Aminoacyl-tRNA synthetases catalyze aminoacylation of tRNAs with their cognate amino acids in two stages. First, the amino acid is activated by ATP to yield the AMP-activated amino acid, with loss of pyrophosphate, followed by transfer of the amino acid onto the tRNA. Malaria parasite genomes encode two different lysyl-tRNA synthetases (KRSs) that play a role in translation in either the cytoplasm (PfKRS1) or in the apicoplast (PfKRS2), while Cryptosporidium parasites and humans encode one copy. We present a selective inhibitor of both Plasmodium and Cryptosporidium lysyl-tRNA synthetase capable of clearing parasites from mouse models of malaria and cryptosporidiosis infection.

By using the luciferase ATP consumption (Kinase-Glo) assay platform with sub-Km substrate concentrations (thus biasing the assay toward identifying ATP-competitive inhibitors), the GlaxoSmithKline malaria actives set of ∼13,000 compounds (the Tres Cantos Antimalarial Set) was screened against recombinant PfKRS1, leading to the discovery of a PfKRS1 inhibitor, compound 2. Compound 2 displayed similar levels of inhibition of PfKRS1 and growth of P. falciparum to cladosporin 1. Compound 2 suffered from high metabolic instability (CLi > 50 mL⋅min−1⋅g−1 in mouse liver microsomes); however, in contrast to cladosporin 1, it was chemically tractable. Screening hit 2 was cocrystallized with PfKRS1 and also binds in the ATP binding pocket, in a similar fashion to cladosporin, although the bicyclic core is rotated 30° with respect to cladosporin. The chromone core stacks between the side chain of F342 on one face and the side chains of H338 and R559 on the other. The ring carbonyl forms an H-bond to the backbone NH of N339, mimicking the N1 of adenine and the O1 OH of cladosporin. The amide carbonyl H-bonds to a highly conserved water molecule coordinated by the side chain of D558 and the backbone NHs of D558 and R559. The cyclohexyl moiety projects into a pocket formed by the side chains of R330, F342, and S344 and the backbone of L555 and G556. This pocket is completed by the substrate lysine and is similar to that occupied by the pyran ring of cladosporin, except that the cyclohexyl ring probes deeper into the pocket.

>EVDPRLYFENRSKFIQDQKDKGINPYPHKFERTISIPEFIEKYKDLGNGEHLEDTILNITGRIMRVSASGQKLRFFDLVGDGEKIQVLANYSFHNHEKGNFAECYDKIRRGDIVGIVGFPGKSKKGELSIFPKETILLSACLHMLPMKYGLKDTEIRYRQRYLDLLINESSRHTFVTRTKIINFLRNFLNERGFFEVETPMMNLIAGGANARPFITHHNDLDLDLYLRIATELPLKMLIVGGIDKVYEIGKVFRNEGIDNTHNPEFTSCEFYWAYADYNDLIKWSEDFFSQLVYHLFGTYKISYNKDGPENQPIEIDFTPPYPKVSIVEEIEKVTNTILEQPFDSNETIEKMINIIKEHKIELPNPPTAAKLLDQLASHFIENKYNDKPFFIVEHPQIMSPLAKYHRTKPGLTERLEMFICGKEVLNAYTELNDPFKQKECFKLQQKDREKGDTEAAQLDSAFCTSLEYGLPPTGGLGLGIDRITMFLTNKNSIKDVILFPTMRPAN[4x]>[3x]MSKPQPIAAANWKSGSPDSLSELIDLFNSTSINHDVQCVVASTFVHLAMTKERLSHPKFVIAAQNAGNADALASLKDFGVNWIVLGHSERRWYYGETNEIVADKVA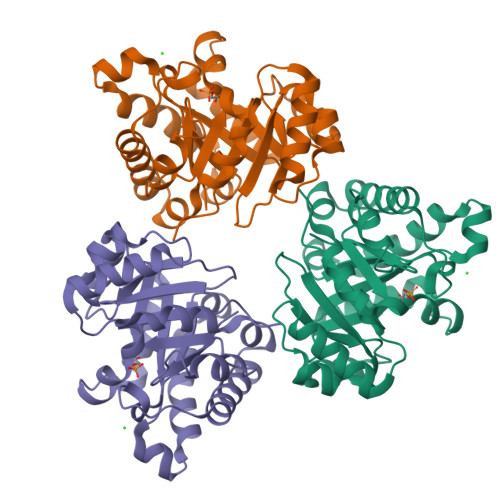AAVASGFMVIACIGETLQERESGRTAVVVLTQIAAIAKKLKKADWAKVVIAYEPVWAIGTGKVLTPQQAQEAHALIRSWVSSKIGADVAGELRILYGGSVNGKNARTLYQQRDVNGFLVGGASLKPEFVDIIKATQ>MGSSHHHHHHSSENLYFQGHSEEAEVGISASTNIPGAQYPQILSGNRVLFRIKAPDAKRVQVDLGKKYDMVREEEGSWAITTDPIVEGFHYYSILIDGVAVCDPASRTFYGMSRMASGIEIPEEGVDYYNLKNVPHGQIRQIRYFSDVTKAWRRAFVYTPAGYDANTSQRYPVLYLQHGGGEDETGWPNQGKMDAIIDNLIAEGKAKPMIVVMDNGYAVDPSA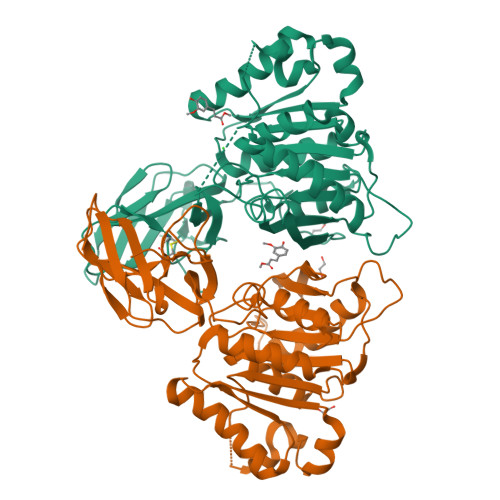SSANSPQGLRGLFQNSALEKVFINEIIPLVDKEFRTIADRDHRAMAGLSMGGFQAFQIAMTNLDKFAYVGGFSGGGIIEQGGDFSKMYNNVWSDVDTFNKRVKLIYLSIGTAEPTNMYQTVNNFHKEFEKAGIKHVYYESPGTSHEWLTWRRSLNQFAELLFK[2x]>[2x]SKETKPLPDYVAWKDADALIVHSDKTLETKRSEFGTSIITPEEKLYIKNNVNTPPESILADRDGWKVEISGVKEPRTLTVAELKTLGLVTAATVLQCSGNGRKYFKDQLTGDQKMSGTPWTVGAAGCVIWSGVPLKAVVDALGGPAEGARFITGTGGEELPAGLDPKLLVVERSVPISNLDNVILA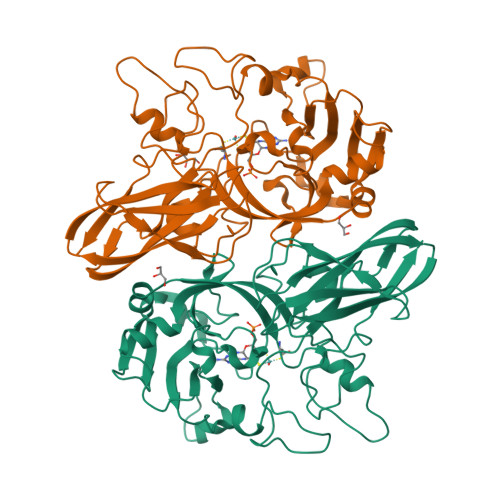WEMNGRPLSLAHGGPLRMVVPGYSGVNNIKYVKAVAMTEVETDAKIQKTSYRVHALGEKGSPDQPSVWEQPVKSWITTPHEAAKAGQVQIAGVAFGGMNACKSVEVSVDGGQTWQEAEFIGPDLGRFAWRVFALSADLARGTYTLVSRATDTEGNVQPEETEMNGAGYGHNGWRAPAVKLTVA>[2x]GPLKPMTFSIYEGQEPSQIIFQFKANPPAVTFELTGETDNIFVIEREGLLYYNRALDRETRSTHNLQVAALDANGIIVEGPVPITIKVKDINDNRPTFLQSKYEGSVRQNSRPGKPFL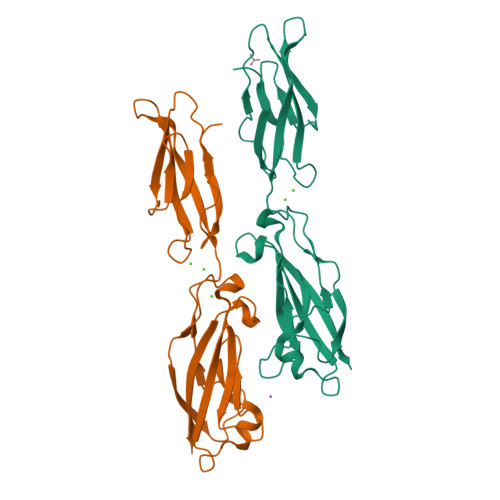YVNATDLDDPATPNGQLYYQIVIQLPMINNVMYFQINNKTGAISLTREGSQELNPAKNPSYNLVISVKDMGGQSENSFSDTTSVDIIVTE>[4x]MIRDTATNTTQTQAAPQQAPAQQFTQAPQEKPMQSTQSQPTPSYAGTGGINSQFTRSGNVQGGDARASEALTVFTRLKEQAVAQQDLADDFSILRFDRDQHQVGWSSLVIAKQISLNGQPVIAVRPLILPNNSIELPKRKTNIVNGMQTDVIESDIDVGTVFSAQYFNRL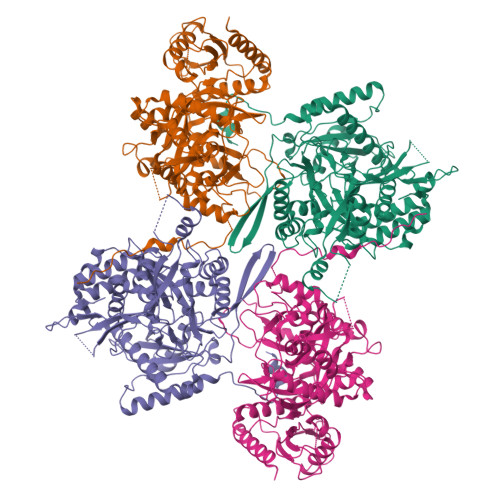STYVQNTLGKPGAKVVLAGPFPIPADLVLKDSELQLRNLLIKSVNACDDILALHSGERPFTIAGLKGQQGETLAAKVDIRTQPLHDTVGNPIRADIVVTTQRVRRNGQQENEFYETDVKLNQVAMFTNLERTPQAQAQTLFPNQQQVATPAPWVASVVITDVRNADGIQANTPEMYWFALSNAFRSTHGHAWARPFLPMTGVAKDMKDIGALGWMSALRNRIDTKAANFDDAQFGQLMLSQVQPNPVFQIDLNRMGETAQMDSLQLDAAGGPNAQKAAATIIRQINNLGGGGFERFFDHTTQPILERTGQVIDLGNWFDGDEKRDRRDLDNLAALNAAEGNENEFWGFYGAQLNPNLHPDLRNRQSRNYDRQYLGSTVTYTGKAERCTYNAKFIEALDRYLAEAGLQITMDNTSVLNSGQRFMGNSVIGNNMVSGQAQVHSAYAGTQGFNTQYQTGPSSFYALEHHHHHH N-(1-ISOPROPYLPIPERIDIN-4-YL)-1-(3-METHOXYBENZYL)-1H-INDOLE-2-CARBOXAMIDE | C25 H31 N3 O2 | 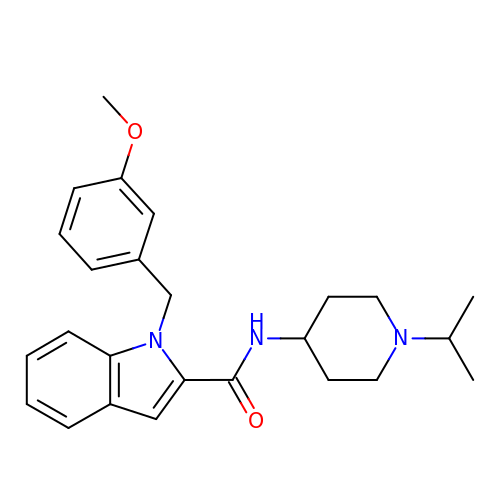GIPCBGDQVGKMPO-UHFFFAOYSA-N>MKRESHKHAEQARRNRL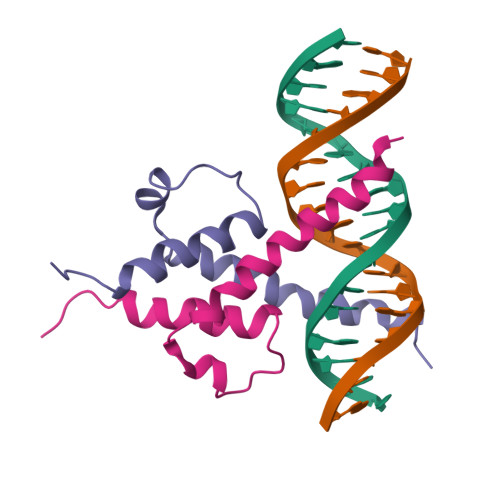AVALHELASLIPAEWKQQNVSAAPSKATTVEAACRYIRHLQQNGST[2x]>MHHHHHHLEPPPSTFQPLCHPLVEEVSKEVDGYFLQHWNFPNEKARKKFVAAGFSRVTCLYFPKALDDRIHFACRLLTVLFLIDDLLEYMSFEEGSAYNEKLIPISRGDVLPDRSIPVEYIIYDLWESMRAHDREMADEILEPVFLFMRAQTDRTRARPMGLGGYLEYRERDVGKELLAALMRFSMGLKLSPSELQRVREIDANCSKHLSVVNDIYSYEKELYTSKTAHSEGGILCTSVQILAQEADVTAEAAKRVLFVMCREWELRHQLLVARLSAEGLETPGLAAYVEGLEYQMSGAELWAQTTLRYSVV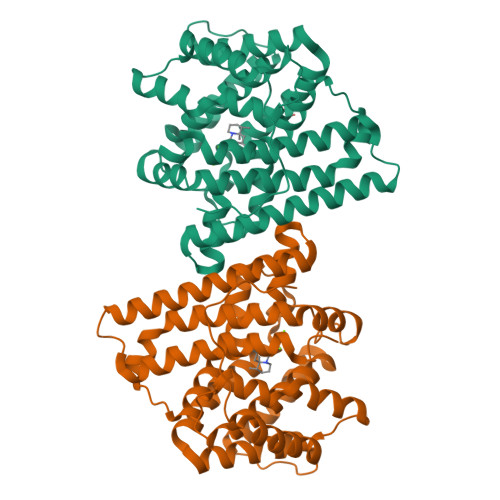VD[4x]>[2x]MVKYEELLKTLENGINSEEGEIRLVRKSQGRFKEEFNFDLSLGSKPLLTLKVFLGRKPYWQPWVEVFGVNPNLRNVFFGSEAERKLYEFLSEHFGRIFVEYFEDKETTYELQKGVPPALSRLGFELLKLGYTYFRDWFIPEGLMEGGHKIQAEKPKTAEAKARHLANLKKEFEEFIGKCEDEGLIKKVKERYNFLEEEAEERCRLAAHHCIHACERYLALCTES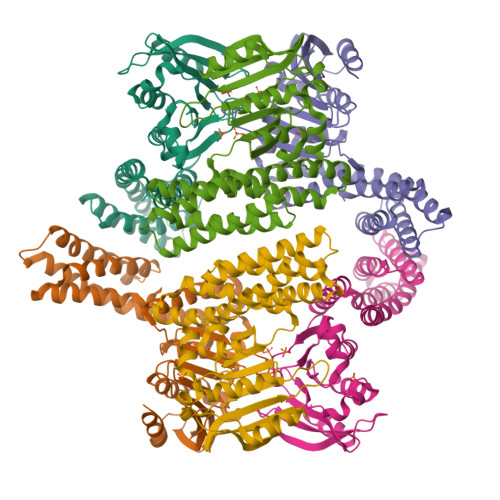SREQRQHAGDCADLCRLAALLLERRSPWAPAACELAARYALACAERCDGDEPLERECAGACRRFVAACAPLL> MPEPSISDLSFTSFVTNDDNLFEETFNFYTKLGFHATRSYVKDNRSDFELTGISTDSIKEIWLESFPLSEVVEASGGRELRKPLQESVGYESEALLGYSPYQSGGVVIKLRLSNHDLEKNNDLPGEVTFFTASIDKLKAKLIEIGAEIIPSKIDLVEFSTRDPMGDVISFSSYPSLNSKKITSPDFFLHPKKEVRSEESIVEQVKSEEGKKKIAIITSGGDAPGMNAAVRAVTRAGIFYGCKVYACYEGYTGLVKGGDMLKELQWQDVRGLLSIGGTIIGTARCKEFRERWGRLQACYNMVSNGIDALVVCGGDGSLTGADLFRKEWPELIKELLGEDKITKEQYETHRNLTIVGLVGSIDNDMCGTDSTIGAYSSLERIIELVDYIDATAASHSRAFVVEVMGRHCGWLGLMSGIATGADYIFIPERPPSESNWKDDLKKVCLRHREKGRRKTTVIVAEGAIDDQLNPITSEEVKDVLVEIGLDTRITRLGHVQRGGAPCAFDRFLATVQGVDAVRAVLESTPAIPSPVISILENKIVRQPLVESVAQTKTVSAAI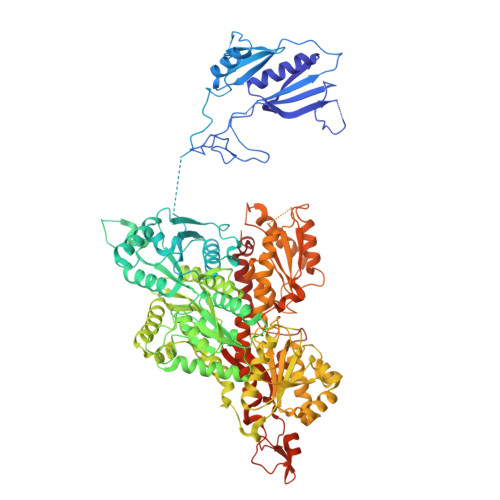EAKDFDKALQLRDQEFATSYENFLSVSKYDDGSYLVPESSRLNIAIIHVGAPTSALNPATRVATLNSLAKGHRVFAIRNGFAGLIRHGAVRELNWIDVEDWHNTGGSEIGTNRSLPSDDMGTVAYYFQQYKFDGLIIIGGFEAFTALYELDAARAQYPIFNIPMCCLPATVSNNVPGTEYSLGSDTCLNTLSGYCDAVKQSASASRRRTFVVEVQGGYSGYLASYAGLITGALAVYTPENPINLQTVQEDIELLTRTYEEDDGKNRSGKIFIHNEKASKVYTTDLIAAIIGEAGKGRFESRTAVPGHVQQGKSPSSIDRVNACRLAIKCCNFIEDANFQVKHNANLSADERHLRFFYDDGVKTSAVSGKSSVIDDNTSVVIGIQGSEVTFTPVKQLWENETHHKWRKGKNVHWEQLNIVSDLLSGRLSIRTT> MPANKLVALTFDDGPDNVLTARVLDKLDKYNVKATFMVVGQRVNDSTAAIIRRMVNSGHEI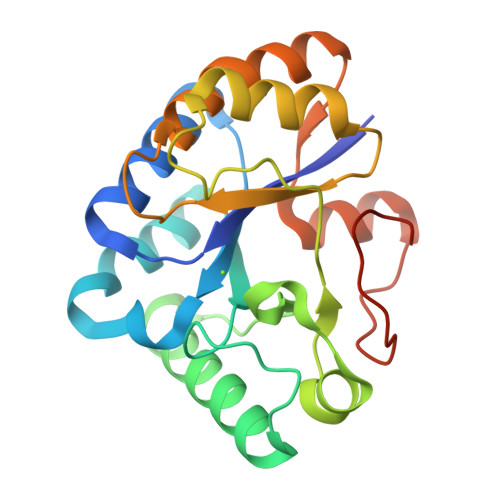GNHSWSYSGMANMSPDQIRKSIADTNAVIQKYAGTTPKFFRPPNLETSPTLFNNVDLVFVGGLTANDWIPSTTAEQRAAAVINGVRDGTIILLHDVQPEPHPTPEALDIIIPTLKSRGYEFVTLTELFTLKGVPIDPSVKRMYNSVPLEHHHHHH> VIPSEPSVRRQPRPAFSVPYAAPESKTQRGLVAICEALLGIDGLGIDDNFFEAGGHSLMLGMLLAQV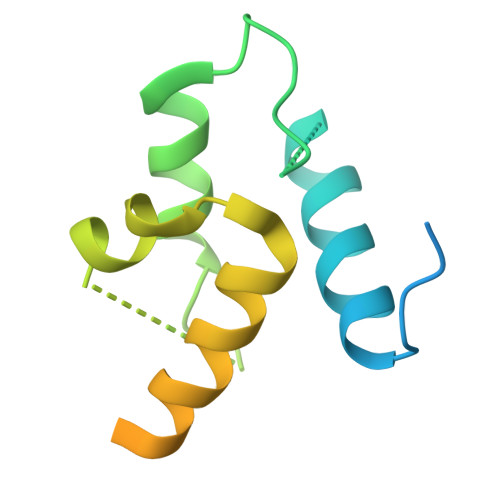QERFAVTLSFFDVMEDASVRALAQLVEQEQQDDGGSALAVLVNDMINEKLSSGLEVLFQGPSSGHHHHHHHHHH> M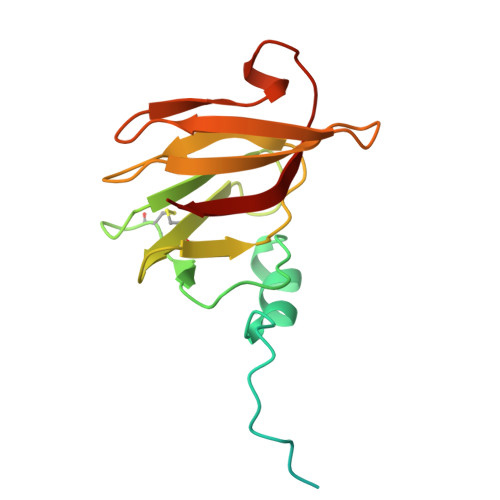ANTSRTRQALMAIAVSVLAAGVTTLGVAHADNGDAVAAAAEMPQAVEDFSYPGAAKIQAETGAILKRGNGHMLMTSCDGSEDIQVMSRTGQKDFCFNVMAKPAYLTLEVPQAYGIWTSADPVKTTIKDTDGTATVINAPANDFTGYGEAGSTGEPTTLIELRVAG> AGIQKDSTGKCGPPPPIDNGDITSFPLSVYAPASSVEYQCANLYQLEGNKRITCRNGQWSEPPKCLHPCVISREI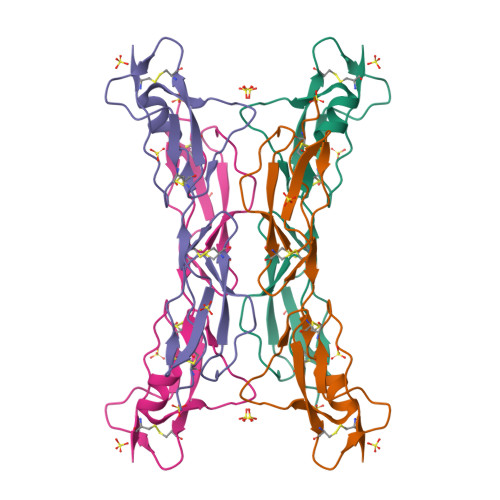MENYNIALRWTAKQKLYSRTGESVEFVCKRGYRLSSRSHTLRTTCWDGKLEYPTCAKR> MTSIEWDEKTFTKFAYLSDPRTRKNLVAYVLTKANLESNKYENTIVIENLEDGSRKFIEDASMPRISPDGKKIAFMRFNEEKKTAQIWVADLKTLSAKKVLEAKNIRSIEWNQDSRRLLAVGFKRREDEDFIFEDDVPAWFDNMGFFDGEKTTFWVIDTEGEEVIEQFEKPRFSSGIWHGDSIVVSVPHRDVIPRYFKYWDIYLWKDGEEEKLFEKVSFYAIDSDGERILLYGKPEKKYVSEHDKIYIYDGEVKGILDDID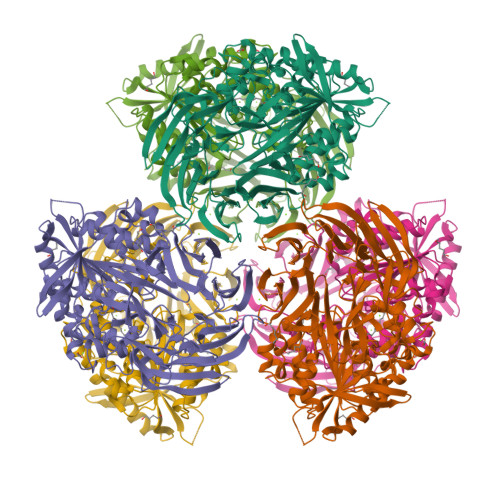REVAQAKIRNGKVYFTLFEEGSVNLYLWDGEVREIAKGKHWIMGFDADERLIYLKETATRPAELYLWDGEERQLTDYNGLIFKKLKTFEPRHFRFKSIDLELDGWYIKPEIKEGEKAPVIVFVHGGPKGMYGYYFKYEMQLMASKGYYIVYVNPRGSNGYSEDFALRVLERTGLEDFQDILNGIEEFLRLEPQADRERIGITGISYGGYMTNWALTQSDLFKAGISENGISYWLTSYAFSDIGLWFDKEVIGDNPLENENYRKLSPLFYAKNVKAPLLLIHSLEDYRCPLDQSLMFYHVLKDLGKEVYIAIFKKGAHGHSIRGSPRHRMKRYKLFMEFFERKLKKYEEGFDVEKILKEEKK Clathrin‐coated pits are formed by the recognition of membrane and cargo by the AP2 complex and the subsequent recruitment of clathrin triskelia. Clathrin cannot recognize membrane or cargo itself and so an adaptor protein binds the membrane, selects the cargo, and associates with clathrin leading to pit formation. The unstructured hinge region contains a clathrin‐box motif (CBM, LLNLD) which binds the N‐terminal domain (NTD) of clathrin heavy chain. The appendage is divided into platform and sandwich subdomain, each with a tyrosine residue previously identified to be important for clathrin binding.

Here, we analysed the cryo‐EM structure of clathrin cages assembled in the presence of β2 hinge‐appendage (β2HA). However in two classes, 15 and 18, distinct density consistent with bound β2HA was observed. In the case of class 15, these densities were in a different location to that shown by our global analysis, on alternate terminal domains within a polyhedral face (Fig EV3A–D). Looking at adjacent polyhedral faces, for a given hub region where 3 terminal domains (from separate triskelia) converge, two terminal domains are engaged in an interaction with a single β2‐appendage leaving one terminal domain unoccupied (Fig EV3C). Interestingly, β2HA density was not present at any of the 4 hubs in the minicoat cage where 3 pentagonal faces join. We extracted and refined the hub regions from each vertex of the minicoat cage particles belonging to Class 15 (Fig EV2), using localized reconstruction within RELION (Ilca et al, 2015). Using this approach we refined a total of 26,624 minicoat hub regions to a global resolution of 9.6 Å (Fig EV4A–I). We also found that separating the hubs according to whether the β2HA density linked terminal domains emerging from two pentagonal faces or from one pentagonal face and one hexagonal face resulted in improved map definition (Fig EV3C and D). These two classes were refined separately to global resolutions of ∼10 Å (10.5 Å for P‐P hubs and 10.1 Å for H‐P hubs, Fig EV4B and C), consistent with the reduced number of particles in each subset. As a control, we performed a similar analysis with the α‐appendage domain which does not bind clathrin. These results predict that residue Tyr 815 on the β2‐appendage makes the largest contribution (14 kJ mol−1) with Asp 812, Gln 804 and Lys 759 contributing at or above a 5 kJ mol−1 threshold at that interface. Interestingly, in our model Lys 140, Lys 189 and Asp 187 form salt bridge contacts with Glu 847, Glu 849 and Arg 904, respectively.

> GGYVAPKAVWLPAVKAKGLEISGTFTHRQGHIYMEMNFTNKALQHMTDFAIQFNKNSFGVIPSTPLAIHTPLMPNQSIDVSLPLNTLGPVMKMEPLNNLQVAVKNNIDVFYFSCLIPLNVLFVEDGKMERQVFLATWKDIPNENELQFQIKECHLNADTVSSKLQNNNVYTIAKRNVEGQDMLYQSLKLTNGIWILAELRIQPGNPNYTLSLKCRAPEVSQYIYQVYDSILKN;>[2x]MAQILPIRFQEHLQLQNLGINPANIGFSTLTMESDKFICIREKVGEQAQVVIIDMNDPSNPIRRPISADSAIMNPASKVIALKAGKTLQIFNIEMKSKMKAHTMTDDVTFWKWISLNTVALVTDNAVYHWSMEGESQPVKMFDRHSSLAGCQIINYRTDAKQKWLLLTGISAQQNRVVGAMQLYSVDRKVSQPIEGHAASFAQFKMEGNAEESTLFCFAVRGQAGGKLHIIEVGTPPTGNQPFPKKAVDVFFPPEAQNDFPVAMQISEKHDVVFLITKYGYIHLYDLETGTCIYMNRIS>[2x]MKYIIEHMEEGFSEWVILEYSQILREVGAENLILSSLPESTTEKDIPQRLLKLGLRWTTKDLKGINEDFKDLELLKDGRVCLLDPRATIDLQPEDATKFDYFVFGGILGDHPPRDRTKELKTAYPNLLISRRLGDKQMTTDTAIRTTQLIIKDRIAFEDIKFIDYPEFRFNKNEATEMPFRYVLDKEGKPILPEGMLDLIKKDSLEHHHHHH

We show that indeed Sfm1 consists of a typical SPOUT domain at the N-terminus flanked by a small C-terminal domain (CTD). Sfm1 exists as a monomer and exhibits a negatively charged surface surrounding the active site unsuitable for RNA binding. Consistently, Sfm1 has no activity towards RNAs but can specifically catalyze the Arg146 methylation of yeast and human S3, and the CTD is critical to the substrate binding and the activity. Sfm1 is the first SPOUT protein that can catalyze protein arginine methylation.

The crystal structure of a C-terminal truncated Sfm1 (Sfm1ΔC: residues 1−204) in apo form was solved by the single-wavelength anomalous dispersion method at 2.0 Å resolution and refined at 1.9 Å resolution, and the crystal structure of the full-length Sfm1 (residues 1−213) in complex with S-adenosyl-homocysteine (SAH) was determined by the molecular replacement method at 2.5 Å resolution. These are two Sfm1 molecules in an asymmetric unit (ASU) in both the apo and SAH-bound Sfm1 structures, which assume almost identical overall structure with a root-mean-square deviation of 1.0 and 0.3 Å, respectively. In the apo Sfm1 structure, all residues of one Sfm1 (molecule A) are well defined; however, a significant portion of the other Sfm1 (molecule B) are undefined owing to poor electron density (residues 79−99, 106−136, 152−162, 185 and 187−189). In both molecules, the C-terminal his-tag (5 residues) and the linker (2 residues) are defined, which are involved in interactions with an adjacent molecule. In the apo Sfm1 structure, the two molecules in the ASU are arranged in a non-symmetric manner (related by a rotation of 145°) and the intermolecular interface involves mainly the C-terminal his-tag, α7 and β9 of the CTD, and the β1-α1 loop of molecule A, and the C-terminal his-tag, the linker, and α7 and β9 of the CTD of molecule B. In addition, the intermolecular interface (between the SPOUT domains) buries about 730 and 1431 Å2 solvent accessible surface in the apo and SAH-bound Sfm1 structures, respectively, which are much smaller than the dimer interfaces (between the SPOUT domains) in the dimeric SPOUT MTases (2 670 Å2 in TrmL, 2 732 Å2 in Nep1 and 2 427 Å2 in TrmD) as calculated using the PISA server. Structural comparison shows that the apo and the SAH-bound Sfm1 assume very similar overall structure (root-mean-square deviation of 1.2 Å for 202 Cα atoms); however, the SAH binding induces some notable conformational changes at the active site. Particularly, on the cofactor binding, the β5-α5 or L2 loop, the following α5 helix, and the β1-α1 loop move towards SAH by about 3.0 Å. These conformational changes lead to formation of a more compact active site and thus several residues of the two loops are either involved in interactions with SAH or in appropriate positions to interact with the substrate.> ADQVDPQLKFAMQRDLGIFPTQLPQYLQTEKLARTQAAAIEREFGAQFAGSWIERNEDGSFKLVAATSGARKSSTLGGVEVRNVRYSLKQLQSAMEQLDAGANARVKGVSKPLDGVQSWYVDPRSNAVVVKVDDGATDAGVDFVALSGADSAQVRIES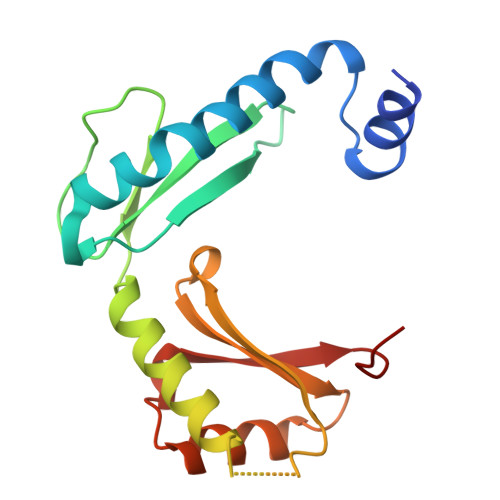SPGKLQTT> GPLGSEDDLYRQSLEIISRYLREQATGSKDSKPLGEAGAAGRRALETLRRVGDGVQRNHETAFQGMLRKLDIKNEDDVKSLSRVMIHVFSDGVTNWGRIVTLISFGAFVAKHLKTINQESCIEPLAESITDVLVRTKRDWLVKQRGWDGFVEFFHVEDLEGG;> DMRPEIWIAQEYRRIGDEFNAY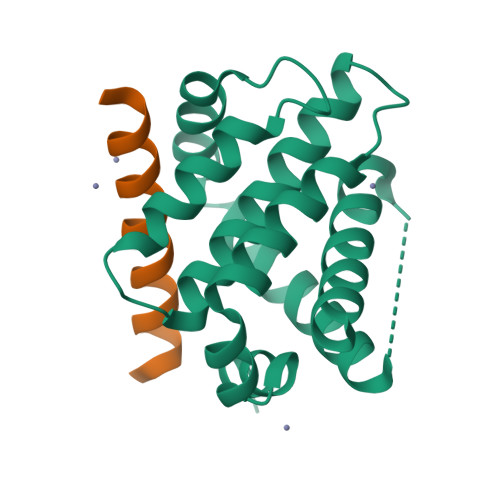YARR>[2x]GSSMDNQDGFILQQVKLSLDDPDSYLSSWNSNDASPCRWSGVSCAGDFSSVTSVDLSSANLAGPFPSVICRLSNLAHLSLYNNSINSTLPLNIAACKSLQTLDLSQNLLTGELPQTLADIPTLVHLDLTGNNFSGDIPASFGKFENLEVLSLVYNLLDGTIPPFLGNISTLKMLNLSYNPFSPSRIPPEFGNLTNLEVMWLTECHLVGQIPDSLGQLSKLVDLDLALNDLVGHIPPSLGGLTNVVQIELYNNSLTGEIPPELGNLKSLRLLDASMNQLTGKIPDELCRVPLESLNLYENNLEGELPASIALSPNLYEIRIFGNRLTGGLPKDLGLNSPLRWLDVSENEFSGDLPADLCAKGELEELLIIHNSFSGVIPESLADCRSLTRIRLAYNRFSGSVPTGFWGLPHVNLLELVNNSFSGEISKSIGGASNLSLLILSNNEFTGSLPEEIGSLDNLNQLSASGNKFSGSLPDSLMSLGELGTLDLHGNQFSGELTSGIKSWKKLNELNLADNEFTGKIPDEIGSLSVLNYLDLSGNMFSGKIPVSLQSLKLNQLNLSYNRLSGDLPPSLAKDMYKNSFIGNPGLCGDIKGLCGSENEAKKRGYVLEGSENLYFQ;>GSSMASANLEGDALHTLRVTLVDPNNVLQSWDPTLVNPCTWFHVTCNNENSVIRVDLGNAELSGHLVPELGVLKNLQYLELYSNNITGPIPSNLGNLTNLVSLDLYLNSFSGPIPESLGKLSKLRFLRLNNNSLTGSIPMSLTNITTLQVLDLSNNRLSGSVPDNGSFSLFTPISFANNLDLCGPVTSHPCPLEGSLENLYFQ[2x];>YVLVPPSGPSMRHN[2x]

Here we demonstrate that HSL1 binds IDA/IDL peptides with high, and CLE peptides with lower affinity, respectively. Ligand sensing capability and receptor activation of HSL1 require a SERK co-receptor kinase. Crystal structures with IDA/IDLs or with CLE9 reveal that HSL1-SERK1 complex recognizes the entire IDA/IDL signaling peptide, while only parts of CLE9 are bound to the receptor. Our work reveals that HSL1 is a receptor for IDA/IDL signaling peptides.

The vastly different binding affinities between IDA/IDLs vs. CLE9 to HSL1 prompted us to determine co-crystal structures of four HSL1-IDA/IDL-SERK1 ternary complexes with: IDA, IDL1, IDL2, and IDL3 (at 2.31 Å, 2.38 Å, 2.20 Å, and 2.70 Å, respectively) and the HSL1-CLE9-SERK1 complex at 2.87 Å. In agreement with our biochemical assays, the crystal structures revealed that all IDA/IDL peptides specifically bind to the peptide-binding surface of HSL1. IDA/IDLs adopt a fully extended conformation in the structure. The co-receptor SERK1 interacts with the C-terminal region of the different IDA/IDL peptides (residues 68-69 in IDA), completing the peptide-binding pocket using its N-terminal loop region. Superposition of the four crystal structures yielded an R.M.S.D of ~0.6 Å comparing 590 Cα atom pairs, with IDL peptides perfectly aligning to each other. Our calorimetry experiments reveal that SERK1 binds HSL1 in the presence of IDA/IDL peptides with a dissociation constant (Kd) of around 15 to 50 nM, indicating that IDA/IDLs promote a high-affinity association between HSL1 and the co-receptor SERK1. Here we report that HSL1 is a bona-fide receptor for IDA/IDL peptides that have evolved a specific binding surface for high-affinity recognition of all IDA/IDL family members.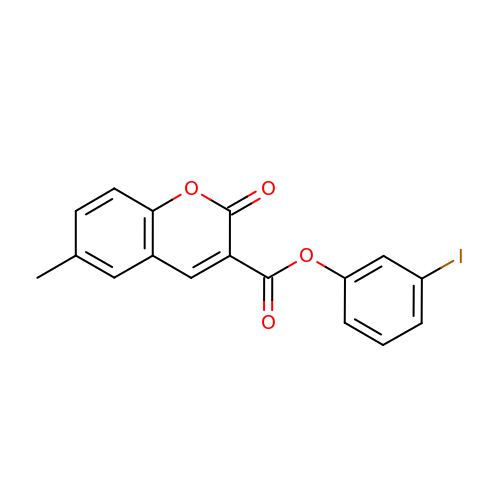(3-iodanylphenyl) 6-methyl-2-oxidanylidene-chromene-3-carboxylate | C17 H11 I O4 | OUKFXYLCMXELAC-UHFFFAOYSA-N>MKYQQLENLESGWKWKYLVKKHREGELITRYIEASAAQEAVDVLLSLENEPVLVNGWIDKHMNPELVNRMKQTIRARRKRHFNAEHQHTRKKSIDLEFIVW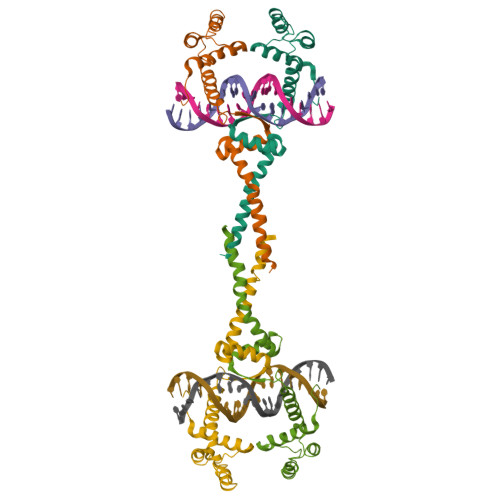QRLAGLAQRRGKTLSETIVQLIEDAENKEKYANKMSSLKQDLQALLGKE[8x]>AQCEATIESNDAMQYNLKEMVVDKSCKQFTVHLKHVGKMAKVAMGHNWVLTKEADKQGVATDGMNAGLAQDYVKAGDTRVIAHTKVIGGGESDSVTFDVSKLTP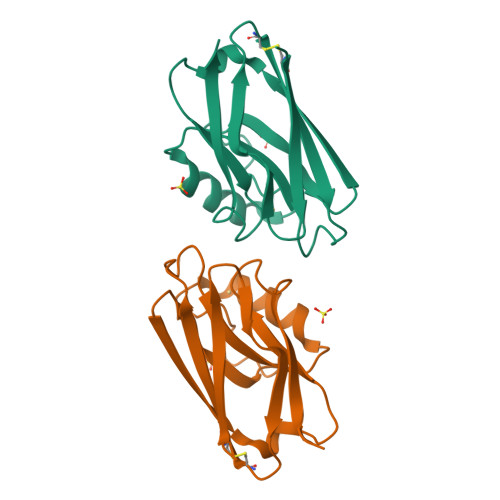GEAYAYFCSFPGHWAMMKGTLKLSN[2x]>GSSPGPYIVRLLNSSLNGCEFPLLTGRTLFVVGQSDALTASGQLPDIPADSFFIPLDHGGVNFEIQVDTDATEIILHELKEGNSESRSVQLNTPIQVGE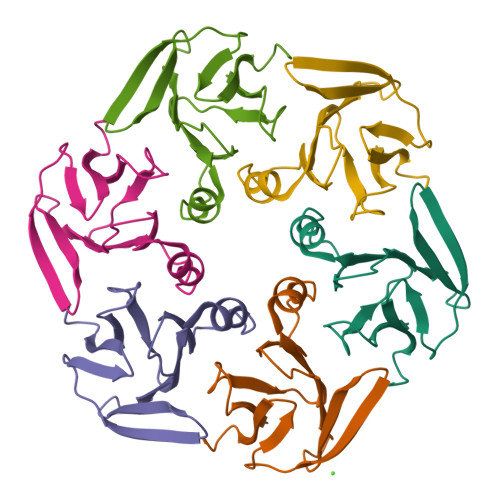LLILIRPESEPW[6x]>MSKSDVFHLGLT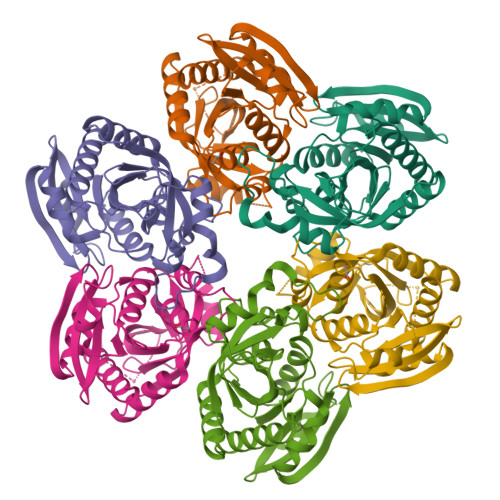KNDLQGAQLAIVPGDPERVEKIAALMDKPVKLASHREFTSWRAELDGKAVIVCSTGIGGPSTSIAVEELAQLGIRTFLRIGTTGAIQPHINVGDVLVTTASVRLDGASLHFAPMEFPAVADFACTTALVEAAKSIGATTHVGVTASSDTFYPGQERYDTYSGRVVRRFKGSMEEWQAMGVMNYEMESATLLTMCASQGLRAGMVAGVIVNRTQQEIPNAETMKQTESHAVKIVVEAARRLL[2x]>MTDPALRAATLLQLHFAFNG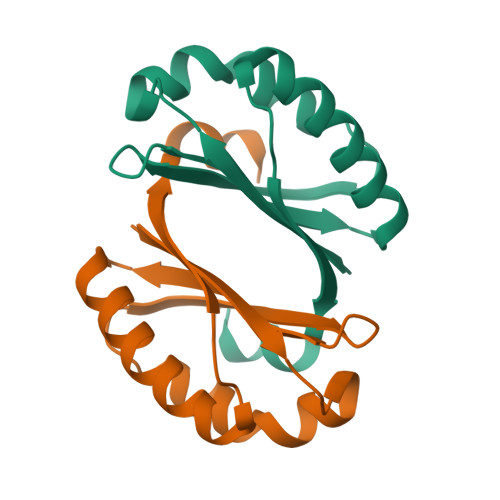PFGDAMAEQLKPLAESINQEPGFLWKVWTESEKNHEAGGIYLFTDEKSALAYLEKHTARLKNLGVEEVVAKVFDVNEPLSQINQAKLAGLCGR[2x]1-(1,2,3-benzothiadiazol-6-yl)-3-[2-(cyclohex-1-en-1-yl)ethyl]urea | C15 H18 N4 O S | 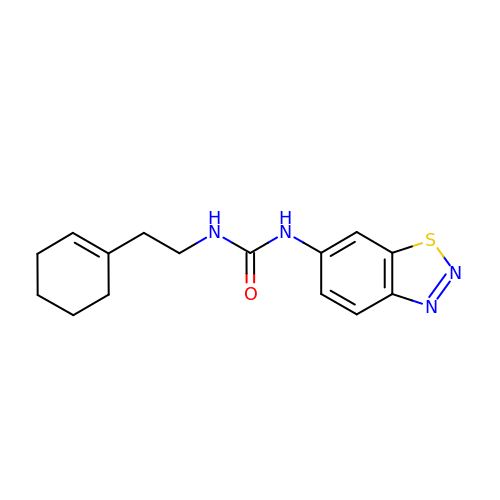GGXCUZHEJUJACD-UHFFFAOYSA-N3-METHOXY-6-[4-(3-METHYLPHENYL)-1-PIPERAZINYL]PYRIDAZINE | C16 H20 N4 O | 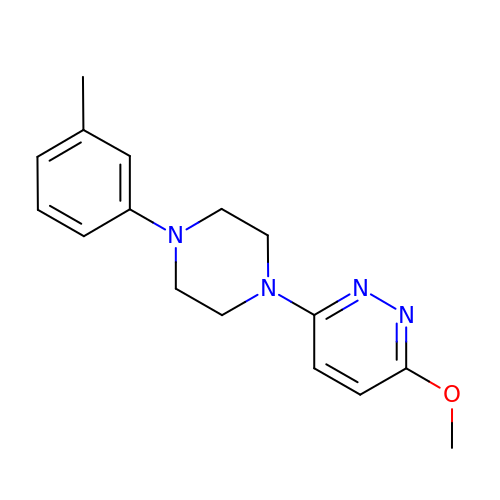DDOAUTHWSCUHQA-UHFFFAOYSA-N> GRQDKMRKEGLQL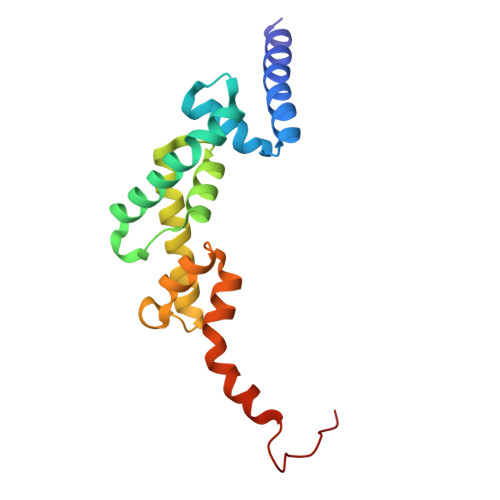VSMIQEGETAGASPEEVFSALQYSGTEVPLQWLRSELSYVLEMVAELAGQQDPELGAFSCQEARKAWLDRHGNLDEAVEECVRARRRKVHELQSLGFGPKEGSLQALFQHGGDVARALTELQRQRLEPFHQRLWDRDPEPTPCWD(3R,4S,5S)-3-[(3-tert-butylbenzyl)amino]-5-[(4,4,7'-trifluoro-1',2'-dihydrospiro[cyclohexane-1,3'-indol]-5'-yl)methyl]tetrahydro-2H-thiopyran-4-ol 1,1-dioxide | C30 H39 F3 N2 O3 S | 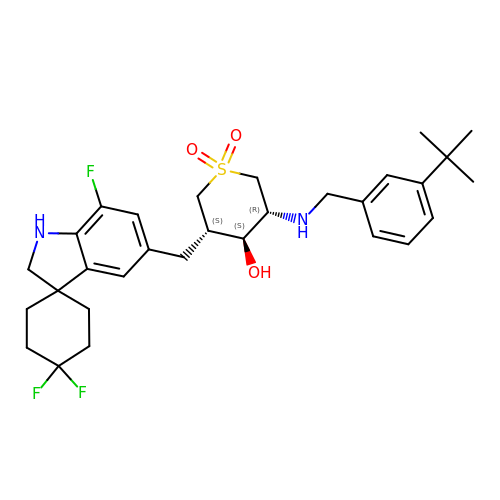YSVPVGYQIWTLEZ-UDZXTKBFSA-N> MQAGPALMSEVASRELRNDTAGVLRR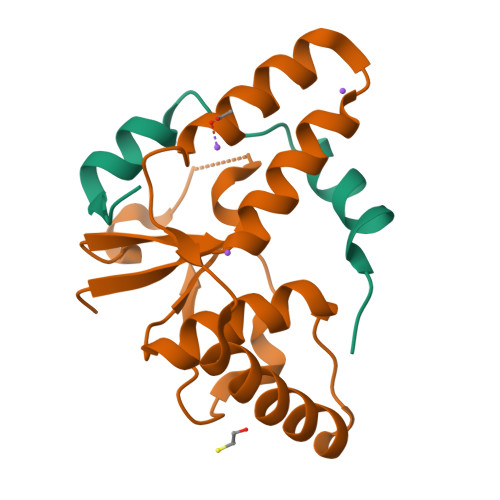VRAGEDVTITVSGRPVAVLTPVRPRRRRWLSKTEFLSRLRGAQADPGLRNDLAVLAGDTTEDLGPIR;> MAHHHHHHVDDDDKMVSTTPAAGVLDTSVFIATESGRQLDEALIPDRVATTVVTLAELRVGVLAAATTDIRAQRLATLESVADMETLPVDDDAARMWARLRIHLAESGRRVRINDLWIAAVAASRALPVITQDDDFAALDGAASVEIIRV>[2x]GHMKQSHFFAHLSRL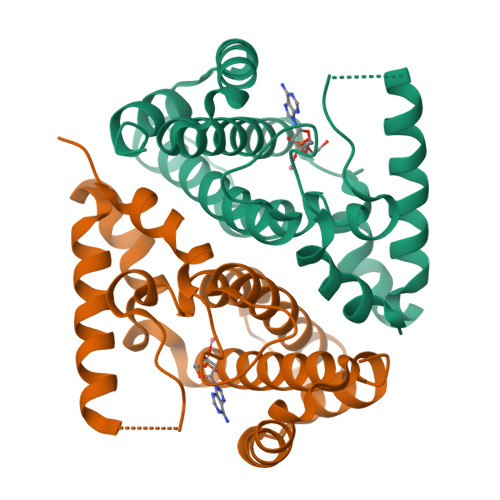KLINRWPLMRNVRTENVSEHSLQVAMVAHALAAIKNRKFGGNVNAERIALLAMYHDASAVLTGDLPTPVKYFNSQIAQEYKAIEKIAQQKLVDMVPEELRDIFAPLIDEHAYSDEEKSLVKQADALCAYLKCLEELAAGNNEFLLAKTRLEATLEARRSQEMDYFMEIFVPSFHLSLDEISQDSPL>[6x]MAPVIPSNTDYPGPHHFEVTFQQSSTAKSATWTYSPLLKKLYCQIAKTCPIQIKVSTPPPPGTAIRAMPVYKKAEHVTDVVKRCPNHELGRDFNEGQSAPASHLIRVEGNNLSQYVDDPVTGRQSVVVPYEPPQVGTEFTTILYNFMCNSSCVGGMNRRPILIIIT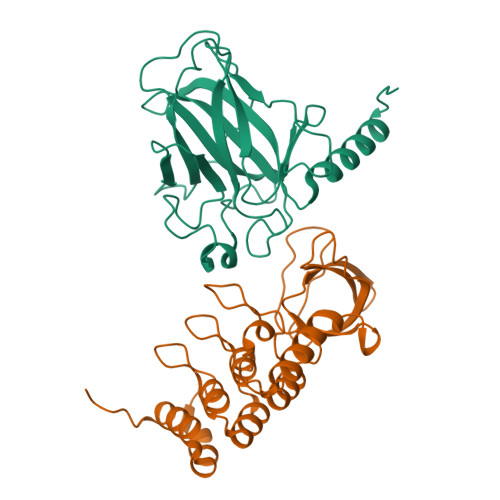LEMRDGQVLGRRSFEGRICACPGRDRKADEDHYREAENLYFQ;>[6x]SMPEITGQVSLPPGKRTNLRKTGSERIAHGMRVKFNPLALLLDSSLEGEFDLVQRIIYEVDDPSLPNDEGITALHNAVCAGHTEIVKFLVQFGVNVNAADSDGWTPLHCAASCNNVQVCKFLVESGAAVFAMTYSDMQTAADKCEEMEEGYTQCSQFLYGVQEKMGIMNKGVIYALWDYEPQNDDELPMKEGDCMTIIHREDEDEIEWWWARLNDKEGYVPRNLLGLYPRIKPRQRSLA> AGSVDTVSLYSGRGANMPFTIMEAESTSNATNGTKLTPNFKPGDYAGEASGRSSVYLDATGEYVEFTLTSPANAFVLRNAVAENTTGTVSIYADGVSKGKFNVSSKFSYLYATPSTLGRLGYDNAPGAGLTAYWLYEDAQLMLDQVYPAGTKIKIQKDAGDVSWIYVDLLETENVAPPQANPDPTKYVAVSASKSIDQALTEFRQDNTKKGIYIPAGEWTINSKIFLYGRATEIVGAGPWYTKLVAPQSQSNTDVGFNISAAANGSTIRDLSAWGNYINRVDGPGKFIDGNGMQNVTVQNIWVEHFVCLYWGVNSSYNTFKNNRIKNTFADGINMTNGSSYNVIDNNYARGTGDDSFALFSATDSGGSYNVGNKYTNLTATNVRRAAAFAVYGGSDNLFQNLYGADTLTYPGITISSYSFGYNTLGFGDQDTVIDGATLDR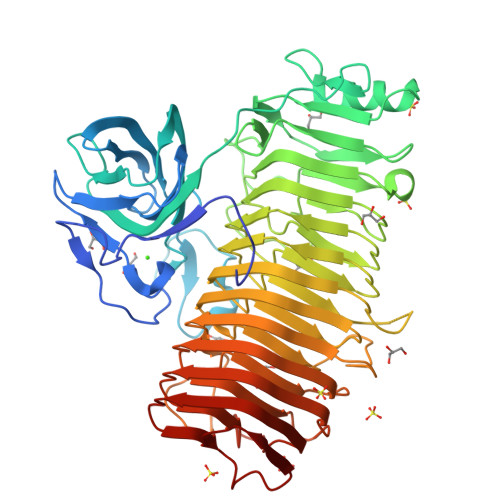TGGDFWTSVGADDKINEYQNFGAIWIYGGDRAIKNILIKNVDINNPVYFGLMFQSMSPNNMVMQNIRVENVNINNPSRYGIKLVVRAEQGQGPAYGGASFTNVKVNNPGISAIYGEAQSPNFTVTRVSGNNW>RKRNRIPLRCTICRKRKVKCDKLRPHCQQCTKTGVAHLCHYMEQTWAEEAEKELLKDNELKKL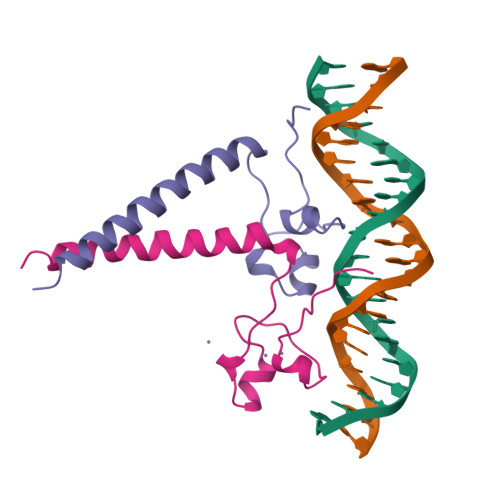RERVKSLEKTLSKVHSSP[2x]>[2x]QDNYRYIKFLTQHYDAKPTGRDYRYCESMMKKRKLTSPCKEVNTFIHDTKNNIKAICGENGNPYGVNFRISNSRFQVTTCTHKGGSPRPPCQYNAFKDFRYIVIACEDGWPVHFDESFISP

Angiogenin (Ang, a 14-kDa protein), an unusual member of the superfamily, is a potent inducer of blood vessel formation that was first isolated from the conditioned medium of cultured HT-29 human colon adenocarcinoma cells based solely on its angiogenic activity. The murine Ang family, over the course of evolution, has expanded to accommodate six members: mAng (the murine orthologue of hAng), mAng-2 (also known as mAngRP or mAng-related protein), mAng-3, mAng-4, mAng-5 and mAng-6 27–31. Experiments have shown that mAng, mAng-3 and mAng-4 have angiogenic activities comparable to that of hAng, whereas mAng-2 is not angiogenic 33–35. The main-chain of both mAng-2 and mAng-3 adopts the familiar α/β fold that is characteristic of other Angs and members of the RNase A family.

The crystal structure of mAng-3 contains a dimer in the asymmetric unit. The CSS for the dimer interface of mAng-3 is 0, suggesting that dimerization is merely a result of crystal packing. The two Zn2+ binding sites in the mAng-3 structure are completely different from each other. One of the zinc ions has only two interactions: one with the hydroxyl group of Tyr14 and the other with a water molecule. The second zinc site has five interactions: one with each of His82 and Glu41, two with water molecules and one with an acetate ion. In the mAng-3 structure, the binding site architecture is very similar to that observed for phosphate and sulfate ions in other Ang structures and both anions ligate the same five P1 subsite residues: Gln12, His13, Lys40, His113 and Phe114. In mAng-3, His113 from chain A is observed in conformation B, whereas the same residue takes on both productive and nonproductive conformations in the other chain. The nonproductive conformation of His113 in chain A of mAng-3 forms a hydrogen bond with an oxygen atom of the nearby sulfate ion via its ND1 atom. In mAng-3, the side-chain of Lys40 points towards the active site of its own protomer. Arg31→Lys31 substitution in mAng-3 is subtle and preserves a surface charge distribution similar to that of hAng.Plastic pollution has become a global environmental challenge, driving interest in enzymatic polyethylene terephthalate (PET) recycling by using polyester hydrolases. Metagenome-derived polyester hydrolases, such as LCC and PHL7, have garnered significant attention due to their high activity at elevated temperatures of up to 70 °C. Their engineering led to the development of optimized variants, including LCCICCG, LCC-A2, Turbo-PETase, and PHL7mut3. , PHL7mut3 has been designed to improve the activity and thermostability of PHL7 by the Q175E, L210T, and D233 K mutations. In this study, the PHL7 wild-type enzyme and the improved PHL7 triple mutant PHL7mut3 were expressed in E. coli and P. pastoris, and their PET-degrading activity under various conditions as well as their thermal stability was assessed. Both the PHL7 and the PHL7mut3 sequences contain three putative N-glycosylation sites (N143, N144, and N161). To assess the impact of mutations and glycosylation on structural folding, we used X-ray crystallography to determine the structures of PHL7mut3, expressed in both E. coli (E_PHL7mut3) and P. pastoris (P_PHL7mut3), as well as a non-glycosylated variant with three additional mutations (P_PHL7mut3_ng), also expressed in P. pastoris.

The crystal structures were resolved at atomic resolution with the highest resolution of 0.89 Å achieved for E_PHL7mut3. The E_PHL7mut3 crystal belonged to the C2 space group, while the P_PHL7mut3 and P_PHL7mut3_ng crystals belonged to the P212121 space group. Structure determination revealed that P_PHL7mut3 and P_PHL7mut3_ng crystallized with one molecule per asymmetric unit, whereas E_PHL7mut3 contained two molecules in the asymmetric unit. In the P_PHL7mut3 structure, electron density supported a single conformation for K233, whereas two conformations were modeled for the same residue in E_PHL7mut3 and P_PHL7mut3_ng. Very weak density indicates multiple conformations of K233 beyond the Cγ-atom in these two structures. We therefore consider the observed flexibility of K233 in the other two structures as characteristic for the enzyme in solution. The difference in the catalytic properties of E_PHL7mut3 and P_PHL7mut3_ng might be caused by the N143Q, N144Q, and N161Q mutations. The C-terminus is quite solvent-exposed, located at a distance of >35 Å to the active site at the opposite side of the protein. Most likely, the additional LE-linker has little influence on the catalytic activity of PHL7.

>MANPYERGPDPTESSIEAVRGPFAVAQTTVSRLQADGFGGGTIYYPTDTSQGTFGAVAISPGFTAGQESIAWLGPRIASQGFVVITIDTITRLDQPDSRGRQLQAALDHLRTNSVVRNRIDPNRMAVMGHSMGGGGALSAAANNTSLEAAIPLQGWHTRKNWSSVRTPTLVVGAELDTIAPVSSHSEAFYNSLPSDLDKAYMELRGASHTVSNTPDTTTAKYSIAWLKRFVDKDLRYEQFLCPAPDDFAISEYRSTCPFLEHHHHHH[2x]>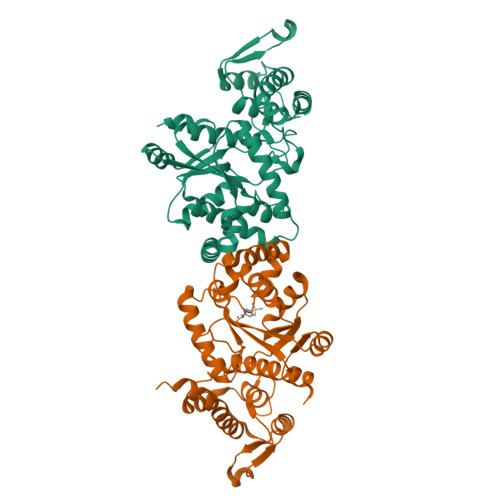[2x]MDEFEMIKRNTSEIISEEELREVLKKDEKSAHIGFEPSGKIHLGHYLQIKKMIDLQNAGFDIGIVLADLQAYLNQKGELDEIRKIGDYNKKVFEAMGLKAKYVYGSEFQLDKDYTLNVYRLALKTTLKRARRSMELIAREDENPKVAEVIYPIMQVNGGHYLGGDVAVGGMEQRKIHMLARELLPKKVVCIHNPVLTGLDGEGKMSSSKGNFIAVDDSPEEIRAKIKKAYCPAGVVEGNPIMEIAKYFLEYPLTIKRPEKFGGDLTVNSYEELESLFKNKELHPMDLKNAVAEELIKILEPIRKRLLEHHHHHH> STAFVDQDKQMANRLNLSPLERSKIEKQYGGATTLAFISNKQQELAQILSRADILKIASYDCAAHALQAVLDCGPMLGKRGFSQSDIVKIAGNIGGAQALQAVLDLESMLGKRGFSRDDIAKMAGNIGGAQTLQAVLDLESAFRERGFSQADIVKIAGNNGGAQALYSVLDVEPTLGKRGFSRADIVKIAGNTGGAQALHTVLDLEPALGKRGFSRIDIVKIAANNGGAQALHAVLDLGPTLRECGFSQATIAKIAGNIGGAQALQMVLDLGPALGKRGFSQATIAKIAGNIGGAQALQTVLDLEP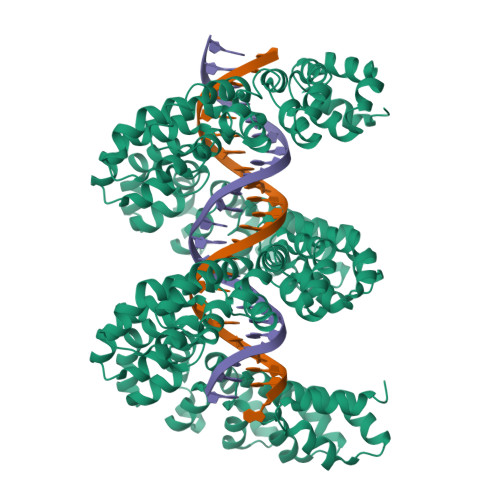ALCERGFSQATIAKMAGNNGGAQALQTVLDLEPALRKRDFRQADIIKIAGNDGGAQALQAVIEHGPTLRQHGFNLADIVKMAGNIGGAQALQAVLDLKPVLDEHGFSQPDIVKMAGNIGGAQALQAVLSLGPALRERGFSQPDIVKIAGNTGGAQALQAVLDLELTLVEHGFSQPDIVRITGNRGGAQALQAVLALELTLRERGFSQPDIVKIAGNSGGAQALQAVLDLELTFRERGFSQADIVKIAGNDGGTQALHAVLDLERMLGDRGFSRADIVNVAGNNGGAQALKAVLEHEATLNERGFSRADIVKIAGNGGGAQALKAVLEHEATLDERGFSRADIVRIAGNGGGAQALKAVLEHGPTLNERGFNLTDIVEMAANSGGAQALKAVLEHGPTLRQRGLSLIDIVEIASNGGAQALKAVLKYGPVLMQAGRSNEEIVHVAARRGGAGRIRKMVAPLLERQGGSEFELENLYFQGELRRQASALE>MNHKVHHHHHHIEGRHMINNKFAVSTISDYTEKINNVKDEEVDDLIKNINKYNYDLFNGTAENQLPDYLNIHEGDVLGYIEIPSINIKLPIYYGTSVDILKKGVGVLEGTSLPVGGENTHSVLSAHTGLANQKLFTDIDKLKDGDVFYLHILKKDLAYKVNQIKVVHPDEIDELKISDDKDYVTLLTCYPYGINTERLLVRGERTDLSP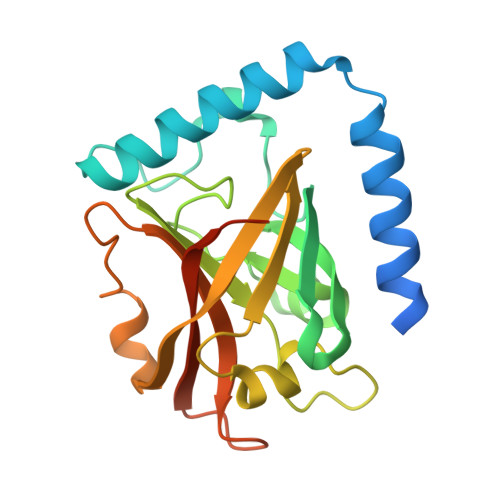SNGAGFSLPST[2x]During activation of a pentameric ligand-gated ion channel (pLGIC), the binding of agonists promotes the opening of a selective ion conduction pore at a distance of more than 50 Å away from the binding sites. Each subunit consists of a predominantly β-stranded extracellular domain and an α-helical transmembrane pore, which interact via an extended interface. Whereas ELIC forms a cation-selective channel with high conductance that is activated with high efficacy by the primary amines cysteamine, propylamine, and GABA, the cation-selective GLIC is activated by protons and inhibited by bulky positively charged compounds that also act as open channel blockers of the nAChR. Our study has identified a cluster of interacting residues located at the β1-β2 turn, the β6-β7 loop and the pre-M1 region of the extracellular domain, and the M2-M3 loop of the pore that exert a strong influence on channel function.

For two cases, the ELIC mutants F116A of the β6-β7 loop and Y258A of the M2-M3 loop, we have grown crystals and determined structures at 3.5 and 3.2 Å, respectively. Both mutants crystallized in the same nonconducting conformation that has been observed in all known ELIC structures. Small structural differences in the vicinity of the respective mutations indicate local rearrangements of protein interactions due to the loss of the bulky aromatic side chains. The data suggests that the mutations, despite their severe phenotype on channel activation, have only a local effect on the protein structure. Neither of the two mutants display ligand-induced channel activity in any of numerous independent recordings. In the background of the mutant R91A, both nonactivatable mutants F116A and Y258A bind agonist and antagonist with similar Keff as the single mutant R91A, thus emphasizing that the mutation has likely not affected ligand binding but instead interfered with channel activation. Similarly, our study has shown that mutations of the corresponding positions in the two prokaryotic channels (T248A, Y250A in GLIC and L256A, Y258A in ELIC) have interfered with activation but not ligand binding, as suggested by the calorimetry experiments of the ELIC mutant Y258A. In both nonconducting conformations, the interactions with the C-terminal part of the M2-M3 loop with the β6-β7 linker remain intact, and the observed nonactivating phenotype of respective mutations (F116A and Y258A in ELIC and F115A and Y250A in GLIC) could thus originate from an interruption of the coupling between the extracellular domain and the pore region.

>[10x]APADNAADARPVDVSVSIFINKIYGVNTLEQTYKVDGYIVAQWTGKPRKTPGDKPLIVENTQIERWINNGLWVPALEFINVVGSPDTGNKRLMLFPDGRVIYNARFLGSFSNDMDFRLFPFDRQQFVLELEPFSYNNQQLRFSDIQVYTENIDNEEIDEWWIRGKASTHISDIRYDHLSSVQPNQNEFSRITVRIDAVRNPSYYLWSFILPLGLIIAASWSVFWLESFSERLQTSFTLMLTVVAYAFYTSNILPRLPATTVIDQMIIAGYGSIFAAILLIIFAHHRQANGVEDDLLIQRCRLAFPLGFLAIGCVLVIRGITL>[3x]GPAVPRMVVLHSLLGMAVLIAIAVLLSTDRKAINIRTVAGAFLIQVALGALVLYVPQGRDMLGEASKTISNVIAYGNNGVDFLFGGLVSEK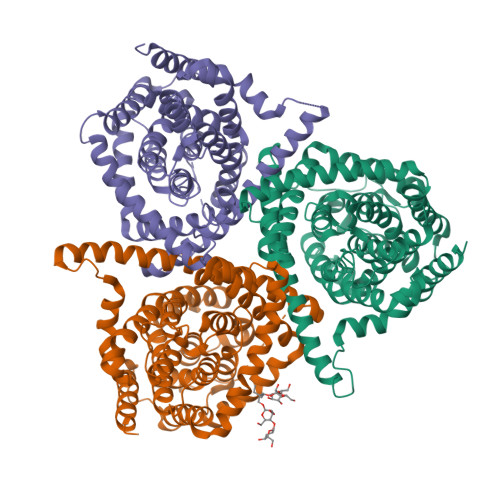MFEVFGGGGFVFALRVLPMIVFFSSLMAVLYYIGVMQLLIKVIGGFLQKMLGTSKAESMSAAALIFVGQTEAPLVVRPYIRRMTESELFAVMSGGLASVAGSVLAGYVQMGVPLPYLIAASFMAAPGGLLFAKLLVPETERTQNDAEVLAENEDEKPTNVIDAAASGAVTGAQIAIAVGASLLAFVALIAMINGIIGGVGGWFGHGDLTLQAILGWLFSPLAWVIGVPWSEAGIAGSLIGQKVVINEFVAYSEFVKYLKPEAAVQLSDTTKAIISFALCGFANLGSIAVLVGGLSIMAPKRRKDVARLGIKAVVAGSLSNLMSAVIAGLFTGLSGASVLG>GAMGSFNSSINNIHEMEIQLKDALEKNQQ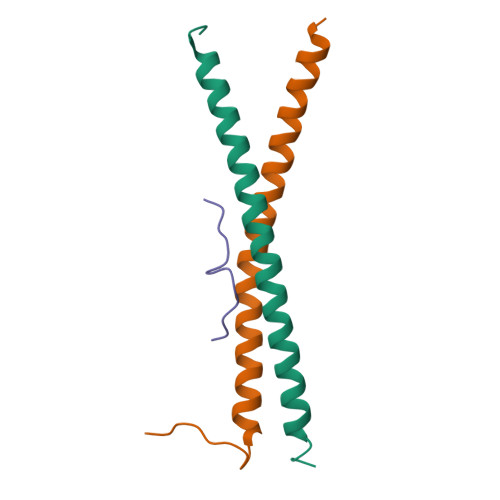WLVYDQQREVYVKGLLAKIFELEKKTETAAHSLP[12x];>DQAQGPPYPTYIPP[6x]> MSKSKVDNQFYSVEVGDSTFTVLKRYQNLKPIGSGAQGIVCAAY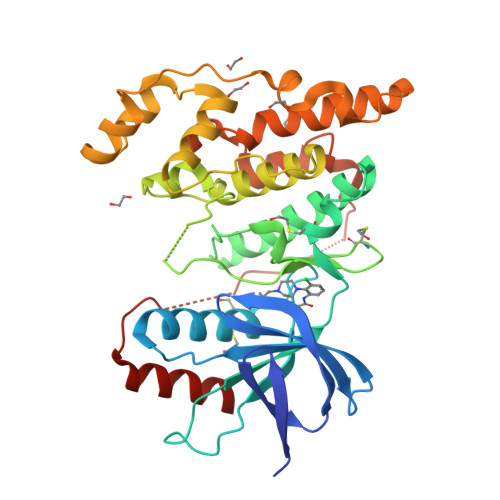DAVLDRNVAIKKLSRPFQNQTHAKRAYRELVLMKCVNHKNIISLLNVFTPQKTLEEFQDVYLVMELMDANLCQVIQMELDHERMSYLLYQMLCGIKHLHSAGIIHRDLKPSNIVVKSDCTLKILDFGLARTAGTSFMMTPYVVTRYYRAPEVILGMGYKENVDIWSVGCIMGEMVRHKILFPGRDYIDQWNKVIEQLGTPCPEFMKKLQPTVRNYVENRPKYAGLTFPKLFPDSLFPADSEHNKLKASQARDLLSKMLVIDPAKRISVDDALQHPYINVWYDPAXXXXXDEREHTIEEWKELIYKEVMNSE> HPTFNKITPNLAEFAFSLYRQLAHQSNSTNIFFSPVSIATAFAMLSLGTKADTHDEILEGLNFNLTEIPEAQIHEGFQELLRTLNQPDSQLQLTTGNGLFLSEGLKLVDKFLEDVKKLYHSEAFTVNFGDTEEAKKQINDYVEKGTQGKIVDLVKELDRDTVFALVNYIFFKGKWERPFEVKDTEEEDFHVDQVTTVKVPMMKRLGMFNIQHCKKLSSWVLLMKYLGNATAIFFLPDEGKLQHLENELTHDIITKFLENEDRRSASLHLPKLSITGTYDLKSVLGQLGITKVFSNGADLSGVTEEAPLK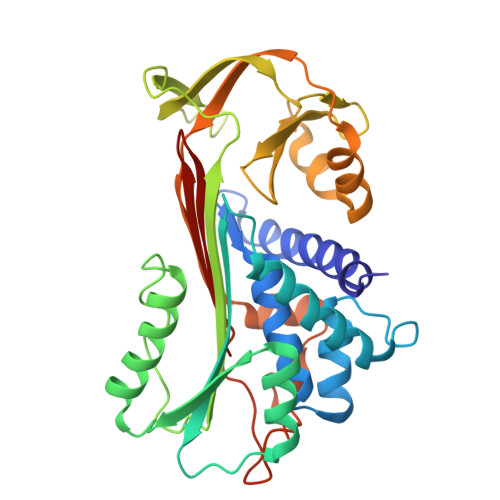LSKAVHKAVLTIDEKGTEAAGAMFL> MDVVDIARWQFGITTVYHFIFVPLTIGLAPLVAIMQTFWQVTGKEHWYRATRFFGTVLLINFAVGVATGIVQEFQFGMNWSEYSRFVGDVFGGPLALEGLIAFFLESVFLGLWIFGWGKIPGWLHTASIWIVAIATNISAYFIIVANSFMQHPVGAEYNPETGRAELTDFWALLTNSTALAAFPHAVAGGFLTAGTFVLGISGWWIIRAHRQAKKAEAEIESKHSMHRPALWVGWWTTVVSSVALFITGDTQAKLMFVQQPMKMASAESLCETATDPNFSILTIGTHNNCDTVTHLIDVPFVLPFLAEGKFTGVTLQGVNQLQAAAEQAYGPGNYSPNLFVTYWSFRAMIGLMLGSLAIAAIAWLLLRKKRTPTGKIARLFQIGSLIAIPFPFLANSAGWIFTEMGRQPWVVHPNPESAGDA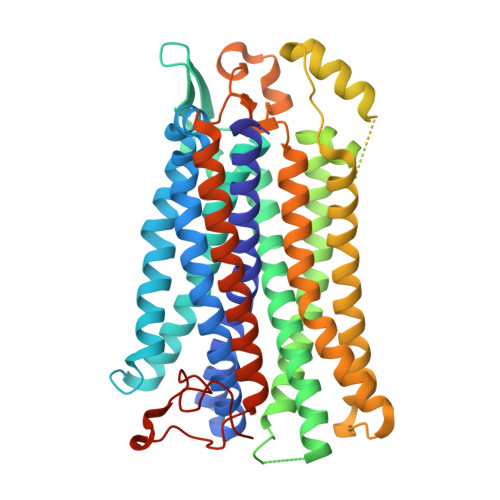RTEMIRMTVDMGVSDHAPWQVWLTLIGFTILYLILFVVWVWLIRRAVLIGPPEEGAPSVEAKTGPATPIGSDMPMTPLQFTAAAPTTREKE> SFSHFLYYLVLIVVIVYGLYKLFTGHGSDINFGKFLLRTSPYMWANLGIALCVGLSVVGAAWGIFITGSSMIGAGVRAPRITTKNLISIIFCEVV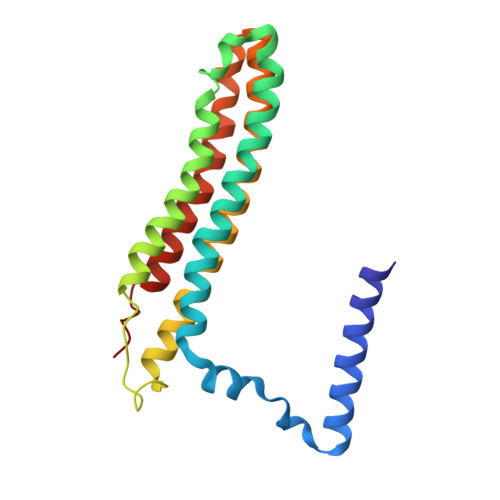AIYGLIIAIVFSSKLTVATAENMYSKSNLYTGYSLFWAGITVGASNLICGIAVGITGATAAISDAADSALFVKILVIEIFGSILGLLGLIVGLLMAGKASEFQ>MNQNLLVTKRDGSTERINLDKIHRVLDWAAEGLHNVSISQVELRSHIQFYDGIKTSDIHETIIKAAADLISRDAPDYQYLAARLAIFHLRKKAYGQFEPPALYDHVVKMVEMGKYDNHLLEDYTEEEFKQMDTFIDHDRDMTFSYAAVKQLEGKYLVQNRVTGEIYESAQFLYILVAACLFSNYPRETRLQYVKRFYDAVSTFKISLPTPIMSGVRTPTRQFSSCVLIECGDSLDSINATSSAIVKYVSQRAGIGINAGRIRALGSPIRGGEAFHTGCIPFYKHFQTAVKSCSQGGVRGGAATLFYPMWHLEVESLLVLKNNRGVEGNRVRHMDYGVQINKLMYTRLLKGEDITLFSPSDVPGLYDAFFADQEEFERLYTKYEKDDSIRKQRVKAVELFSLMMQERASTGRIYIQNVDHCNTHSPFDPAIAPVRQSNLCLEIALPTKPLNDVNDENGEIALCTLSAFNLGAINNLDELEELAILAVRALDALLDYQDYPIPAAKRGAMGRRTLGIGVINFAYYLAKHGKRYSDGSANNLTHKTFEAIQYYLLKASNELAKEQGACPWFNETTYAKGILPIDTYKKDLDTIANEPLHYDWEALRESIKTHGLRNSTLSALMPSETSSQISNATNGIEPPRGYVSIKASKDGILRQVVPDYEHLHDAYELLWEMPGNDGYLQLVGIMQKFIDQSISANTNYDPSRFPSGKVPMQQLLKDLLTAYKFGVKTLYYQNTRDGAEDAQDDLVPSIQDDGCESGACKI[2x];>MAYTTFSQTKNDQLKEPMFFGQPVNVARYDQQKYDIFEKLIEKQLSFFWRPEEVDVSRDRIDYQALPEHEKHIFISNLKYQTLLDSIQGRSPNVALLPLISIPELETWVETWAFSETIHSRSYTHIIRNIVNDPSVVFDDIVTNEQIQKRAEGISSYYDELIEMTSYWHLLGEGTHTVNGKTVTVSLRELKKKLYLCLMSVNALEAIRFYVSFACSFAFAERELMEGNAKIIRLIARDEALHLTGTQHMLNLLRSGADDPEMAEIAEECKQECYDLFVQAAQQEKDWADYLFRDGSMIGLNKDILCQYVEYITNIRMQAVGLDLPFQTRSNPIPWINTWLVSDNVQVAPQEVEVSSYLVGQIDSEVDTDDLSNFQL[2x]

pmcRibonucleotide reductases (RNRs) are essential enzymes in DNA biosynthesis and repair. They convert all four ribonucleotides (CDP, UDP, ADP, and GDP) into the corresponding deoxyribonucleotides. Finally, class I RNRs employ a second subunit (β) for radical storage, necessitating a long-range RT (~35 Å) between α and β subunits for thiyl radical generation. Subsequent research by Stubbe, Nocera, and Bennati using unnatural amino acids and spectroscopy confirmed that RT occurs over long distances and involves proton-coupled electron transfer (PCET) and the formation of multiple transient amino acid radical species.

Our 2.6-Å resolution structure of a trapped α2β2 complex was obtained using wild-type protein, N3CDP, dATP as the specificity effector, and ATP as the activity effector. Our overall structure is consistent with the asymmetry observed in the prior cryo-EM structure: β2 is primarily contacting α and not α′. Refinement of an “SN-CDP” (sulfur–nitrogen–CDP) adduct to Cys225 shows that the adduct fits the density with geometric parameters that agree with the spectroscopic data. Collectively, these observations indicate that α′ is postturnover and α is midturnover. As expected, we find two ATP molecules bound in the allosteric activity sites in the N-terminal cone domain of α. Despite the presence of these two ATP molecules, there are no substantial changes in the cone domain’s interactions with β compared to the α2β2 structure without ATP. Instead of a polar residue in direct contact with Y356β, water molecules are positioned to contact Y356β, supporting the proposal that water molecules are the direct proton donors/acceptors of Y356β and thus play a direct role in PCET, consistent with electron nuclear double resonance (ENDOR) and electron paramagnetic resonance (EPR) spectroscopies and DFT studies. With our improved resolution, we can identify that there are two water channels, which we will refer to as pink and yellow channels, that connect bulk solvent with Y356β. Notably, in this midturnover structure, we observe that the E623α side chain has flipped away from Y731α, and a water molecule (Water1014 in Chain B) has taken the place of glutamate’s carboxylate.A class I chitinase from the carnivorous sundew plant Drosera adelae was successfully expressed in the methylotrophic yeast Pichia pastoris and efficiently purified using a chitin affinity column. Enzymatic activity assays revealed that the enzyme showed a specific activity of 235.3 ± 10.2 U·mg−1. In D. adelae chitinase, a characteristic tyrosine cluster consisting of Tyr174, Tyr199, and Tyr201 formed a unique structural feature that enabled recognition of the (GlcNAc)4 substrate. The hevein domain structures further indicated that the tyrosine cluster (Tyr41, Tyr43, Tyr50) in D. adelae chitinase may be involved in hydrogen bonding and CH/π interactions with (GlcNAc)3.

Crystallization of wild‐type and E167Q catalytic mutant chitinases yielded needle‐like microcrystals. X‐ray diffraction experiments were performed, and high‐resolution datasets were obtained at 1.73 Å and 1.57 Å, respectively. Structural analysis of diffraction data revealed that only the catalytic domain could be resolved in both crystal forms.

> DVSSIITSQIFNQMLLHRNDNACPANGFYSYQAFINAARKFSGFGTTGDTNTRKNELAAFFGQTSHETTGGWSTAPDGPYAWGYCFKQQQGNPGDYCVPSSTYPCAPGKKYYGRGPIQISYNYNYGLCGAAINQPLLSNPGLVASDADISFETAIWFWMTPQGNKPSCHAVATGQWNPSSADQAAGRVPGYGVITNIINGGVECGQGEKAEVANRIGFYQRYCSIFGISPGQNLDCYNQRPFS> HMSIQEIQKEIAQIQAVIAGIQKYIYTMTGGSGGSGGGGSGGSGGMSIEE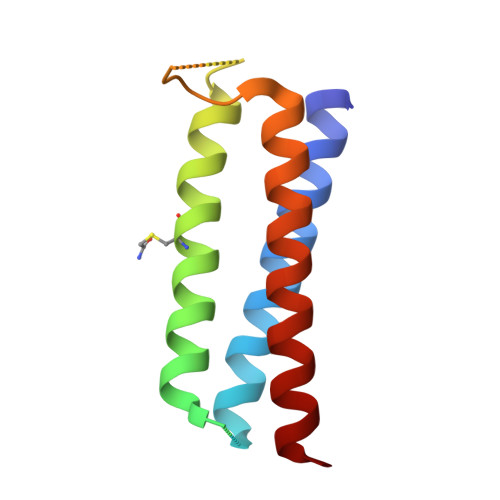IQKQIAAIQCQIAAIQKQIYAMTGSGGGGSGGSGGGGSGMSIEEIQKQIAAIQEQILAIYKQIMAMVT>MASMTGGQQMGRGSMSRDPLPFFPPLYLGGPEITTENCEREPIHIPGSIQPHGALLTADGHSGEVLQMSLNAATFLGQEPTVLRGQTLAALLPEQWPALQAALPPGCPDALQYRATLDWPAAGHLSLTVHRVGELLILEFEPTEAWDSTGPHALRNAMFALESAPNLRALAEVATQTVRELTGFDRVMLYKFAPDATGEVIAEARREGLHAFLGHRFP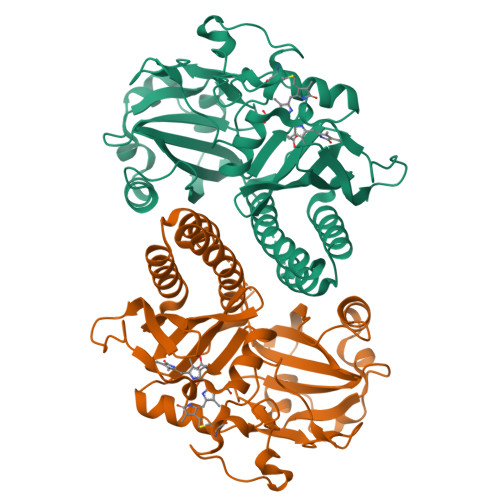ASDIPAQARALYTRHLLRLTADTRAAAVPLDPVLNPQTNAPTPLGGAVLRATSPMHMQYLRNMGVGSSLSVSVVVGGQLWGLIACHHQTPYVLPPDLRTTLEYLGRLLSLQVQVKEALEHHHHHH[2x]> AETVESCLAKPHTENSFTNVWKDDKTLDRYANYEGCL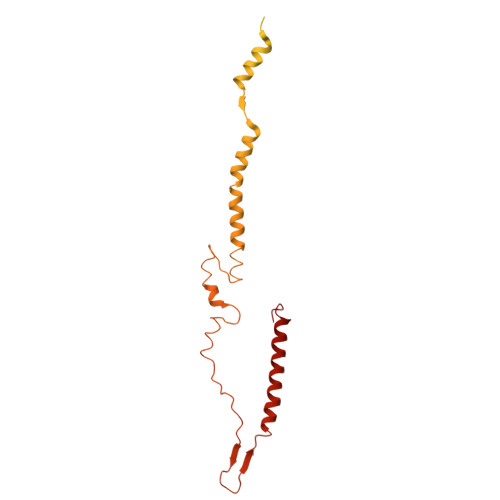WNATGVVVCTGDETQCYGTWVPIGLAIPENEGGGSEGGGSEGGGSEGGGTKPPEYGDTPIPGYTYINPLDGTYPPGTEQNPANPNPSLEESQPLNTFMFQNNRFRNRQGALTVYTGTVTQGTDPVKTYYQYTPVSSKAMYDAYWNGKFRDCAFHSGFNEDPFVCEYQGQSSDLPQPPVNAGGGSGGGSGGGSEGGGSEGGGSEGGGSEGGGSGGGSGSGDFDYEKMANANKGAMTENADENALQSDAKGKLDSVATDYGAAIDGFIGDVSGLANGNGATGDFAGSNSQMAQVGDGDNSPLMNNFRQYLPSLPQSVECRPFVFGAGKPYEFSIDCDKINLFRGVFAFLLYVATFMYVFSTFANILRNKES2-amino-N-[4-methoxy-3-(trifluoromethyl)phenyl]-4-methyl-3-[2-(methylamino)quinazolin-6-yl]benzamide 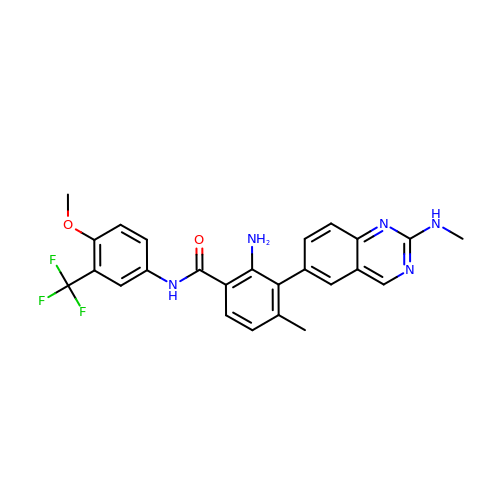| C25 H22 F3 N5 O2 | NYVUSSXLPQHLMH-UHFFFAOYSA-N> MTTTQPTLALPGQLLGPISKYQPGPGTHVHESNLYSSLLGTVHVTQPARAPGPVKRLNRITPAPTPAELPTISVSAARPAGSAASGLVTGRKREILPEVGNIVLCRVIRITPRQAVVTILVCGDTVLDAEWQGLIRVQDIRATEKDRVKVYESFRPGDIVRAEVISLGDQANYYLSTARNELGVILATSEAGNTMYPVSWR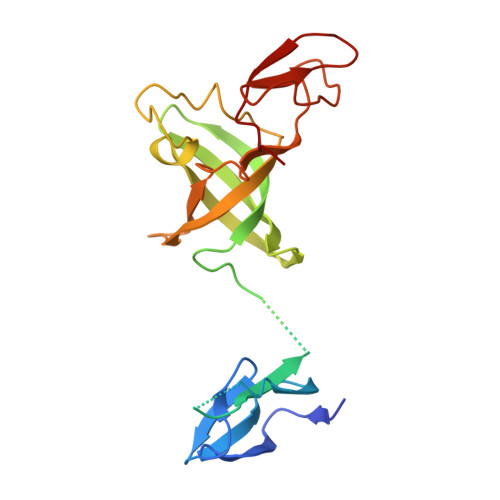EYRDPITGLTELRKVAKPY> VTPGAILVTHPL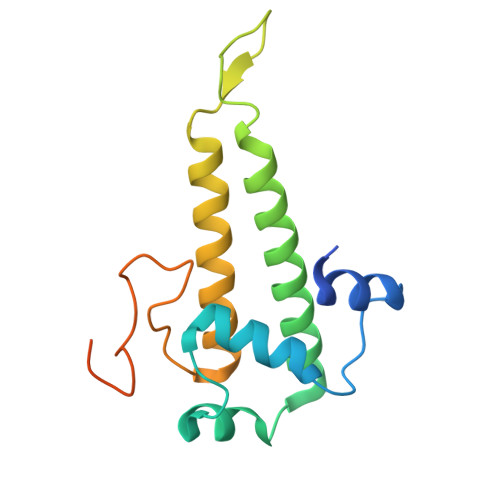ESYYNQFLDGLPTSELEELEIEFVAMCIGFPRSQNNFVNALLDLSTIEVYTIRTSVKEILRLDKLNKESIENRQVTKVEDITMNMNYIGDIKDELVTEVKKLARILKLPVLDNLYVSYDDVEGRIGANGLLEPLNRGSGFGSYLTGYTVR> MSGAFGCGSYRSVVAGTQNVPRRMTFYPSAYELIQLHKAHREVIRHFYVRDKIF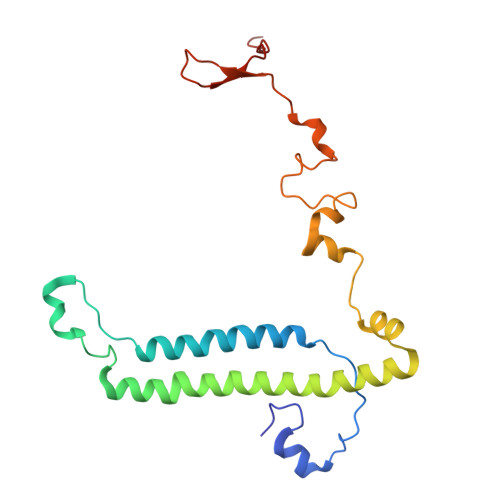DNKFPGNALANGLFKFVPNRRENYHMRELMESIRRRSIWMHRIKQQREINAKVVENMEVKYGKKAAASMLCFTTPDSNAYFAPHRYQDVANSWPNYWQHPSVNHVVPKPRWRRHRELGGITRVEDPFAVQASDY>[6x]MPIVVTQAHIDRVGIAADLLDASPVSLQVLGRPTAINTVVIKTYIAAVMELASKQGGSLAGVDIRPSVLLKDTAIFTKPKAKSADVESDVDVLDTGIYSVPGLARKPVTHRWPSEGIYSGVTALMGATGSGKSITLNEKLRPDVLIRWGEVAEAYDELDTAVHISTLDEMLIVCIGLGALGFNVAVDSVRPLLFRLKGAASAGGIVAVFYSLLTDI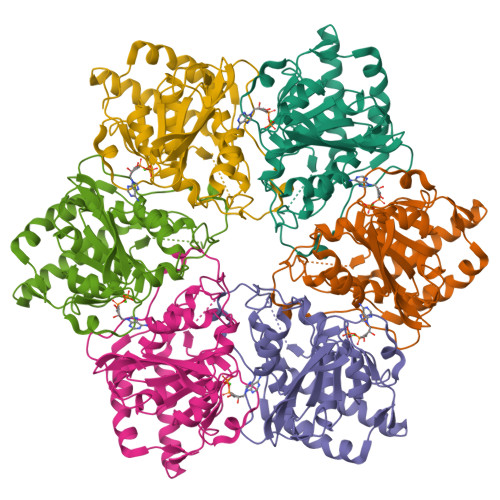SNLFTQYDCSVVMVVNPMVDAEKIEYVFGQVMASTVGAILCADGNVSRTMFRTNKGRIFNGAAPLAADTHMPSMDRPTSMKALDHTSIASVAP>[3x]MGSSHHHHHHENLYFQGEVKQQSESELKHYYNKPILERKNVTGFKYTDEGKHYLEVTVGQQHSRITLLGSDKDKFKDGENSNIDVFILREGDSRQATNYSIGGVTKSNSVQYI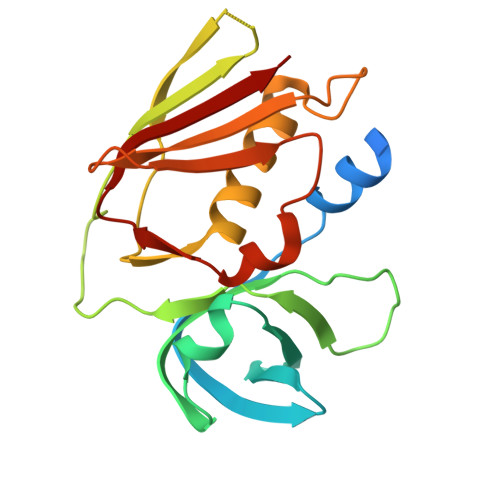DYINTPILEIKKDNEDVLKDFYYISKEDISLKELDYRLRERAIKQHGLYSNGLKQGQITITMNDGTTHTIDLSQKLEKERMGESIDGTKINKILVEMK> GEESRNTTVLDTTTTLQSSGFGRAFFGEAFNDLKTLMRRYQLYGQLLLSVTTDKDIDHCMFTFPCLPQGLALDIGSAGSPHEIFNRCRDGIIPLIASGYRFYRGDLRYKIVFPSNVNSNIWVQHRPDRRLEGWSAAKIVNCDAVSTGQGVYNHGYASHIQI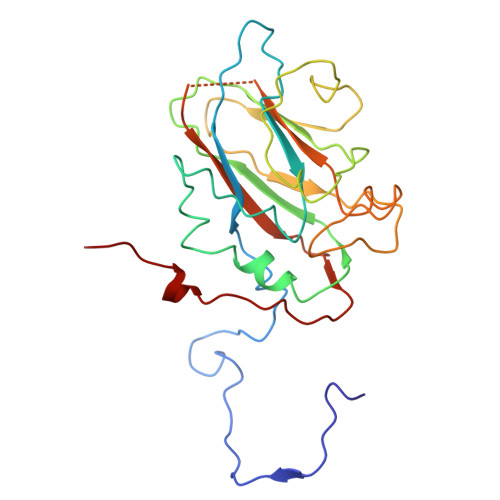TRVNNVIELEVPFYNATCYNYLQAFNASSAASSYAVSLGEISVGFVNKPVTIYYSIGDGMQFSQWVGYQPMMILDQLPAPVV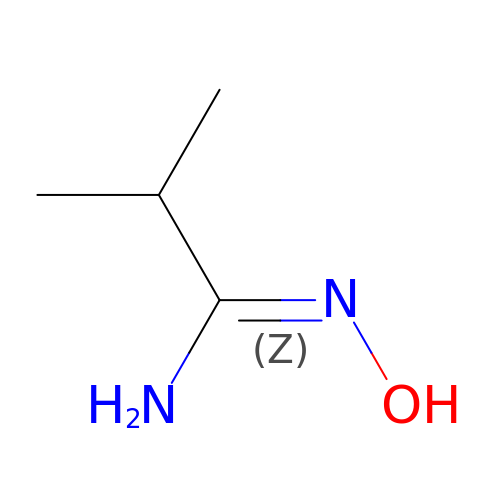2-methyl-~{N}'-oxidanyl-propanimidamide | C4 H10 N2 O | JHRDEHLFNLLCQS-UHFFFAOYSA-N>[4x]MKMASNDANPSDGSAANLVPEVNNEVMALEPVVGAAIAAPVAGQQNVIDPWIRNNFVQAPGGEFTVSPRNAPGEILWSAPLGPDLNPYLSHLARMYNGYAGGFEVQVILAGNAFTAGKIIFAAVPPNFPTEGLSPSQVTMFPHIIVDVRQLEPVLIPLPDVRNNFYHYNQSNDSTIKLIAMLYTPLRANNAGEDVFTVSCRVLTRPSPDFDFIFLVPPTVESRTKPFTVPILTVEEMTNSRFPIPLEKLFTGPSGAFVVQPQNGRCTTDGVLLGTTQLSPVNICTFRGDVTHIAGSRNYTMNLASLNWNNYDPTEEIPAPLGTPDFVGKIQGVLTQTTKGDGSTRGHKATVYTGSAPFTPKLGSVQFSTDTENDFETHQNTKFTPVGVIQDGSTTHRNEPQQWVLPSYSGRNVHNVHLAPAVAPTFPGEQLLFFRSTMPGCSGYPNMDLDCLLPQEWVQHFYQEAAPAQSDVALLRFVNPDTG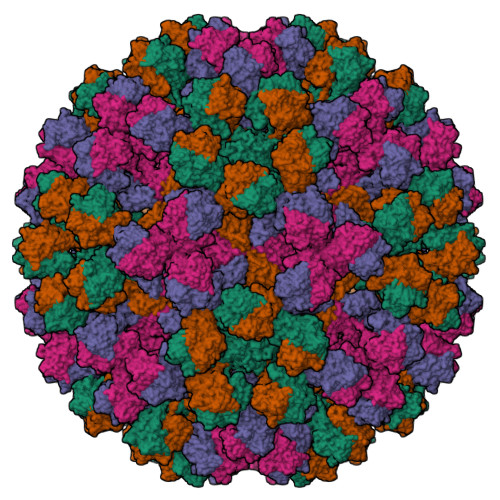RVLFECKLHKSGYVTVAHTGQHDLVIPPNGYFRFDSWVNQFYTLAPMGNGTGGRRAL> MPPRPSSGELWGIHLMPPRILVECLLPNGMIVTLECLREATLITIKHELFKEARKYPLHQLLQDESSYIFVSVTQEAEREEFFDETRRLCDLRLFQPFLKVIEPVGNR;> YQQDQVVKEDNIEAVGKKLHKYNTQFQEKSREYDRLYEEYTRTSQEIQMKRTAIEAFNETIKIFEEQCQTQERYSKEYIEKFKREGNEKEIQRIMHNYDKLKSRISEIIDSRR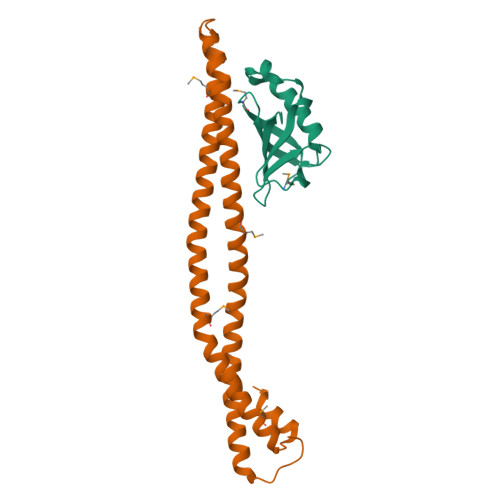RLEEDLKKQAAEYREIDKRMNSIKPDLIQLRKTRDQYLMWLTQKGVRQKKLNEWLGN> MGSSHHHHHHSSGRENLYFQGHMADRQLLHTAHIPVRWGDMDSYGHVNNTLYFQYLEEARVAWFETLGIDLEGAAEGPVVLQSLHTYLKPVVHPATVVVELYAGRLGTSSLVLEHRLHTLEDPQGTYGEGHCKLVWVRHAENRSTPVPDS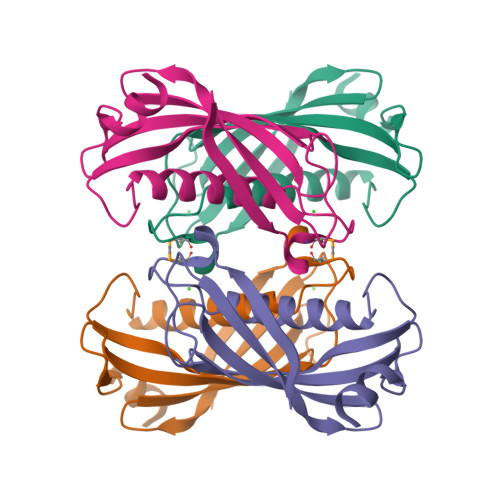IRAAIAGS> MTLEVIGISVLWLFLFGYIIVASIDFGAGFFSVYSHWANQQHILHRIIQRYLSPVWEVTNVFLVFFFVGIVGFFPKTAYYYGSILLVPASIAIVLLAIRGSYYAFHTYGETERNWYLLAYGLTGLFIPASLSIVLTISEGGFVEENAAGVALDYGKLFASPLSWSVVLL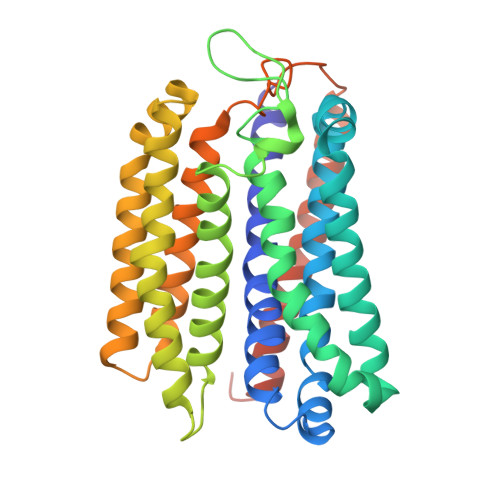SVTSVLYISAVFLTYYADAAGDEQARALLRRYALLWSGPTMLSALLIIYQLRYHNPEHYDNLWNVAWMLVISFLFFVITVWLLGRQRRFGWAFIALLFQYAFAFYAYGISHYPYLLYPYLTIYDGFTNETMAMALIVAFIAGLLLLIPSLYLLMRLFLFNKAYVKGKWEGGKG INOSINIC ACID 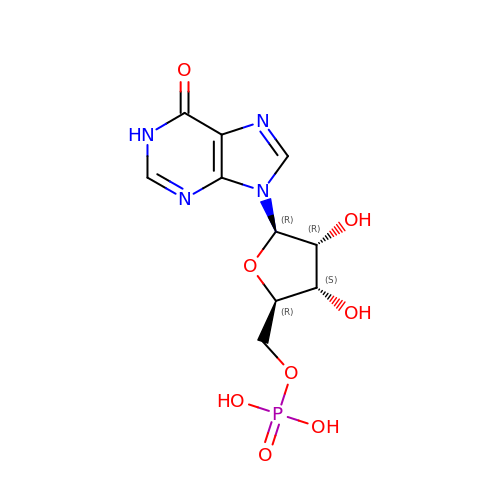| C10 H13 N4 O8 P | GRSZFWQUAKGDAV-KQYNXXCUSA-N> GSHMASMTGGQQMGRGSMSLTEEKPIRPIANFSPSIWGDQFLIVDNQVEQGVEQIVKDLKKEVRQLLKEALDIPMKHANLLKLVDEIQRLGISYLFEQEIDHALQHIYETYGDNWSGARSSLWFRLMRKQGYFVTCDVFNNHKDESGVFKQSLKNHVEGLLELYEATSMRVPGEIILEDALVFTQSHLSIIAKDTLSINPALSTEIQRALKKPLWKRLPRIEAVQYIPFYEQQDSHNKTLIKLAKLEFNLLQSLHREELSQLSKWWKAFDVKNNAPYSRDRIVECYFWALASRFEPQYSRARIFLAKVIALVTLIDDIYDAYGTYEELKIFTEAIERWSITCLDMIPEYMKPIYKLFMDTYTEMEEILAKEGKTNIFNCGKEFVKDFVRNLMVEAQWANEGHIPTTEELDSVAVITGGANLLTTTCYLGMSDIVTKEAFEWAVSEPPLLRYK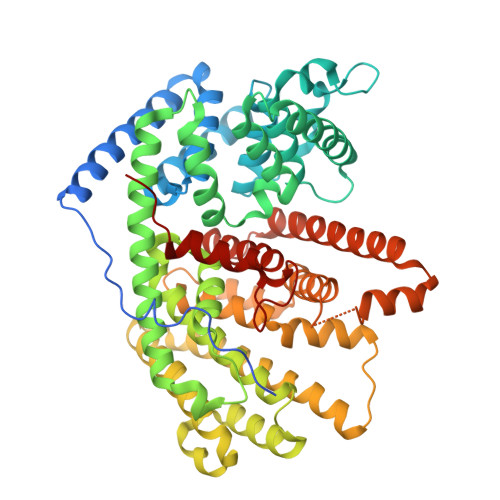GILGRRLNDLAGHKEEQERKHVSSSVESYMKEYNVSEEYAKNLLYKQVEDLWKDINREYLITKTIPRPLLVAVINLVHFLDVLYAAKDAFTAMGEEYKNLVKSLLVYPMSI> SNAMASQIDQYAVFGNPINHSKSPFIHTLFARQTQQSMIYTAQCVPVDGFTEAAKHFFAQGGRGCNVTVPFKEEAYRFADRLTERARLAGAVNTLKKLDDGEILGDNTDGEGLVQDLLAQQVLLKGATILLIGAGGAARGVLKPLLDQQPASITVTNRTFAKAEQLAELVAAYGEVKAQAFEQLKQSYDVIINSTSASLDGELPAIDPVIFSSRSVCYDMMYGKGYTVFNQWARQHGCAQAIDGLGMLVGQAAE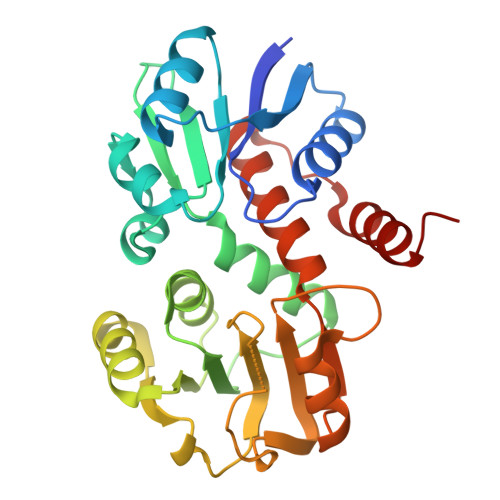SFMLWRGLRPGTKQILRELRKNLEGAL>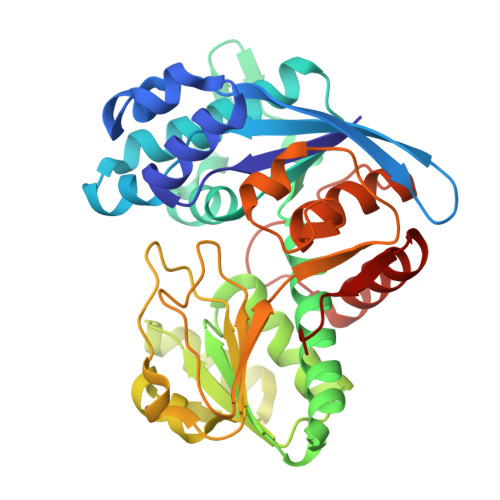 MFGLIGHLTSLEQARDVSRRMGYDEYADQGLEFWSSAPPQIVDEITVTSATGKVIHGRYIESCFLPEMLAARRFKTATRKVLNAMSHAQKHGIDISALGGFTSIIFENFDLASLRQVRDTTLEFERFTTGNTHTAYVICRQVEAAAKTLGIDITQATVAVVGATGDIGSAVCRWLDLKLGVGDLILTARNQERLDNLQAELGRGKILPLEAALPEADFIVWVASMPQGVVIDPATLKQPCVLIDGGYPKNLGSKVQGEGIYVLNGGVVEHCFDIDWQIMSAAEMARPERQMFACFAEAMLLEFEGWHTNFSWGRNQITIEKMEAIGEASVRHGFQPLALAI>[4x]NLFVALYDFVASGD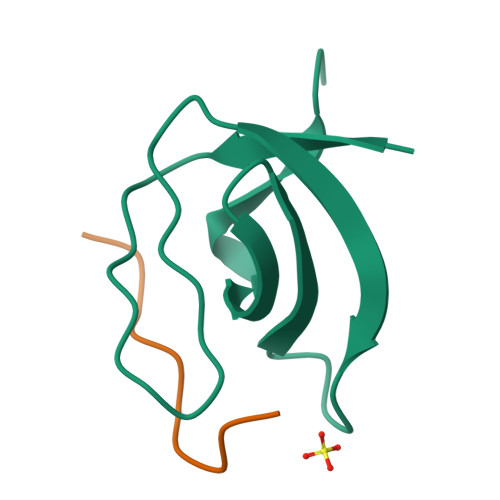NTLSITKGEKLRVLGYNHNGEWCEAQTKNGQGWVPSNYITPVNS;>[4x]XAPSYSPPPPP>MAKFPKNFMFGYSWSGFQFEMGLPGSEVESDWWVWVHDKENIASGLVSGDLPENGPAYWHLYKQDHDIAEKLGMDCIRGGIEWARIFPKPTFDVKVDVEKDEEGNIISVDVPESTIKELEKIANMEALEHYRKIYSDWKERGKTFILNLYHWPLPLWIHDPIAVRKLGPDAAPAGWLDEKTVVEFVKFAAFVAYHLDDLVDMWSTMNEPNVVYNQGYINLASGFPPGFLSFEAAEKAKFNLIQAHIGAYDAIKEYSEKSVGVIYAFAWHDPLAEEYKDEVEEIRKKDYEFVTILHSKGKLDWIGVNYYSRLVYGAKDGHLVPLPGYGFMSERGGFAKSGRPASDFGWEMYPEGLENLLKYLNNAYELPMIITENGMADAADRYRPHYLVSHLKAVYNAMKEGADVRGYLHWSLTDNYEWAQGFRMRFGLVYVDFETKKRYLRPSALVFREIATQKEIPEELAHLADLKFVTRK[4x]

β-Glucosidase from Pyrococcus furiosus (BGLPf) is a hyperthermophilic tetrameric enzyme which can degrade cellooligosaccharides to glucose under hyperthermophilic conditions and thus holds promise for the saccharification of lignocellulosic biomass at high temperature. Hyperthermophilic archaeal BGL (BGLPf; family 1) has also been isolated from P. furiosus and holds significant potential for the complete saccharification of cellulose at high temperature when combined with EGPh. BGLPf exhibits high hydrolytic activity towards cellooligosaccharides at high temperatures. The thermostability of BGLPf is affected by its oligomeric structure.

Therefore, in order to disrupt these intersubunit interactions, we constructed a BGLPf mutant (R170A/R220A/Y227F) in which Arg170, Arg220 and Tyr227 were substituted by Ala, Ala and Phe, respectively. This three-point mutation of BGLPf is referred to as BGLPf-M3. Crystal structural analysis showed that the BGLPf-M3 crystals belonged to space group C2, which is different from that of BGLPf-WT. Diffraction data were improved to 1.70 Å resolution and the structure was refined. The four monomers of BGLPf-M3 in the asymmetric unit were named subunits P, Q, R and S. The root-mean-square (r.m.s.) deviations of the Cα-atom positions (1–471) among subunits P, Q, R and S are less than 0.27 Å. Furthermore, the r.m.s. deviations of the Cα-atom positions (1–471) of subunits P, Q, R and S of BGLPf-M3 compared with subunit A of BGLPf-WT are between 0.27 and 0.31 Å. These results indicate that the overall structure of the monomer is not influenced by the mutations. Molecules of glycerol, which was used as a cryoprotectant, were observed in the putative active site of each of the four monomers of BGLPf-M3 and were also observed in the BGLPf-WT crystal structure. The electron-density map of BGLPf-M3 revealed cis-type peptide bonds at two sites in each subunit: between Pro224 and Pro225 and between Trp410 and Ser411. The crystal structure of BGLPf-M3 exhibits higher resolution than that of BGLPf-WT and also shows several noteworthy interactions between sub­units R and S. the PQ and RS dimers are distinct from each other, even though the PQ dimer of BGLPf-M3 is similar to the AC dimer of BGLPf-WT. Two types of alternative dimers (PQ and RS) are formed in BGLPf-M3, with residues Arg381, Tyr382, Arg448, Glu449 and Glu459 controlling dimer formation.> QYSSNTQQGRTSIVHLFEWRWVDIALECERYLAPKGFGGVQVSPPNENVAIHNPFRPWWERYQPVSYKLCTRSGNEDEFRNMVTRCNNVGVRIYVDAVINHMCGNAVSAGTSSTCGSYFNPGSRDFPAVPYSGWDFNDGKCKTGSGDIENYNDATQVRDCRLSGLLDLALGKDYVRSKIAEYMNHLIDIGVAGFRIDASKHMWPGDIKAILDKLHNLNSNWFPEGSKPFIYQE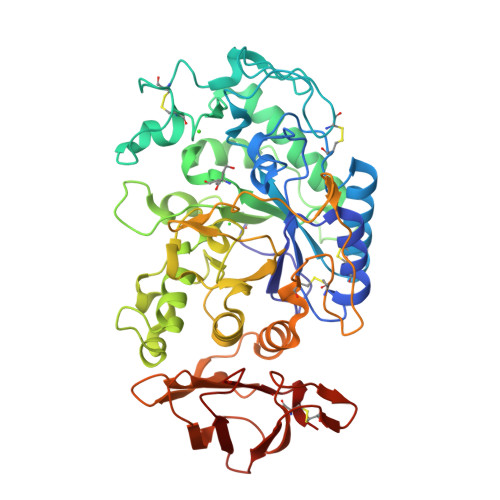VIDLGGEPIKSSDYFGNGRVTEWKYGAKLGTVIRKWNGEKMSYLKNWGEGWGFMPSDRALVFVDNHDNQRGHGAGGASILTFWDARLYKMAVGFMLAHPYGFTRVMSSYRWPRYFENGKDVNDWVGPPNDNGVTKEVTINPDTTCGNDWVCEHRWRQIRNMVNFRNVVDGQPFTNWYDNGSNQVAFGRGNRGFIVFNNDDWTFSLTLQTGLPAGTYCDVISGDKINGNCTGIKIYVSDDGKAHFSISNSAEDPFIAIHAESKL>ATCYCRTGRCATRESLSGVCEIS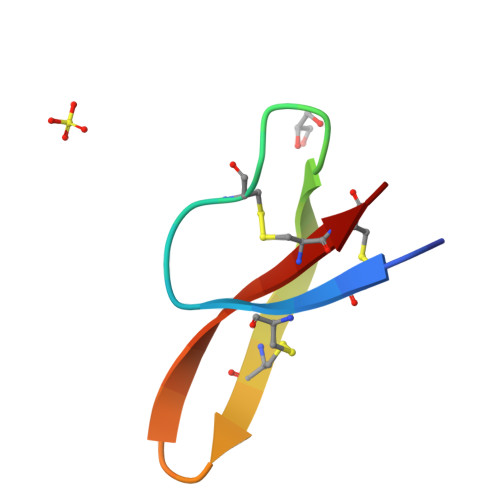GRLYRLCCR[4x]6-(1,3-dimethyl-5-oxidanyl-pyrazol-4-yl)carbonyl-1,5-dimethyl-3-(2-methylphenyl)quinazoline-2,4-dione 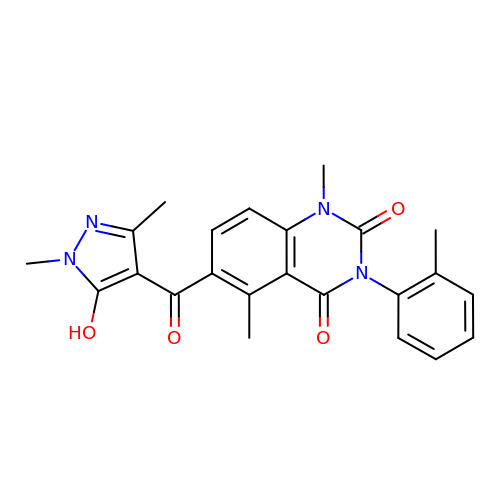| C23 H22 N4 O4 | YKHYFGVAUPZAFT-UHFFFAOYSA-N> MGSLVCVGTGLQLAGQISVLSRSYIEHADIVFSLLPDGFSQRWLTKLN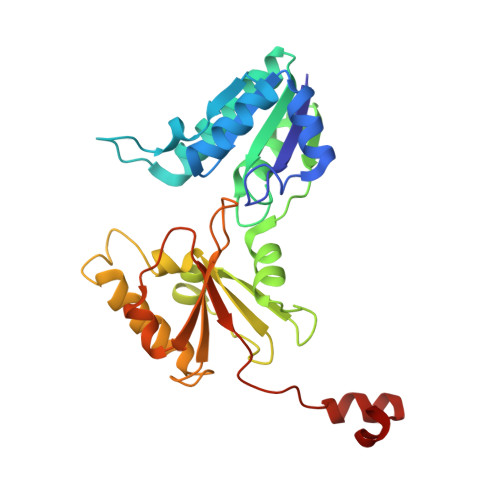PNVINLQQFYAQNGEVKNARDTYEQMVNAILDAVRAGKKTVCALYGHPGVFACVSHMAITRAKAEGFSAKMEPGISAEACLWADLGIDPGNSGHQSFEASQFMFFNHVPDPTTHLLLWQIAIAGEHTLTQFHTSSDRLQILVEQLNQWYPLDHEVVIYEAANLPIQAPRIERLPLANLPQAHLMPISTLLIPPAKKLEYNYAILAKLGIGPEDLG> GDITHMEKLGDICFSLRYVPTAGKLTVVILEAKNLKKMDVGGLSDPYVKIHLMQNGKRLKKKKTTIKKNTLNPYYNESFSFEVPFEQIQKVQVVVTVLDYEKIGKNDAIGKVFVGYNSTGAELRHWSDMLANPRRPIAQWHTLQVEEEVDAML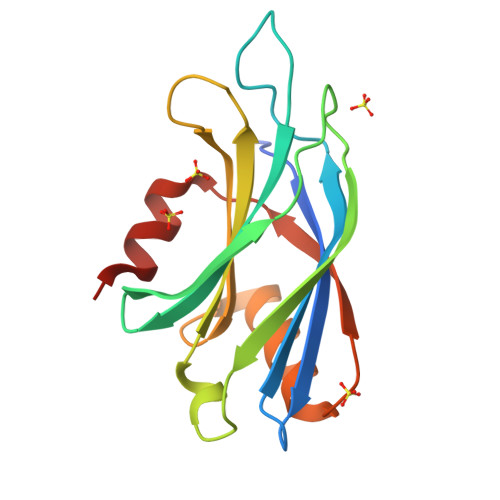AVKK>[2x]SMGEAICSALPTIPYHKLADLRYLSRGASGTVSSARHADWRVQVAVKHLHIHTPLLDSERKDVLREAEILHKARFSYILPILGICNEPEFLGIVTEYMPNGSLNELLHRKTEYPDVAWPLRFRILHEIALGVNYLHNMTPPLLHHDLKTQNILLDNEFHVKIADFGLSKWRMMSLSQSRSSKSAPEGGTIIYMPPENYEPGQKSRASIKHDIYSYAVITWEVLSRKQPFEDVTNPLQIMYSVSQGHRPVINEESLPYDIPHRARMISLIESGWAQNPDERPSFLKCLIELEPVLRTFEEITFLEAVIQLKKTKLQSV

RIPK2 is a caspase recruitment domain (CARD) containing kinase that has been implicated in nucleotide binding and oligomerization domain 1 and 2 (NOD1 and NOD2) signaling. NOD-RIPK2 interactions result in activation of nuclear factor κB (NF-κB) and mitogen-activated protein (MAP) kinase pathways to promote the transcription of pro-inflammatory cytokines. This signaling pathway potentially plays a crucial role in an array of pathological conditions including inflammatory bowel disease, Crohn’s disease and multiple sclerosis. Herein, we report the design of receptor-interacting protein kinase 2 (RIPK2) inhibitors based on pan-kinase inhibitor regorafenib that aim to engage basic activation loop residues Lys169 or Arg171.

We report development of CSR35 that displayed >10-fold selective inhibition of RIPK2 versus VEGFR2, the target of regorafenib. Two RIPK2 molecules were found in the asymmetric unit. As expected, CSR35 was bound to a DFG-out conformation and retained interactions characteristic of most type II inhibitors. The pyridine nitrogen and hydrogen of the amide formed hydrogen bonds with the hinge region (Met98). The urea was engaged in hydrogen bonds with the catalytic residue Glu66 and the backbone NH of Asp164 of the DXG motif. But most interestingly, one of the monomers revealed that Lys169 of the activation loop forms an ionic–ionic interaction with the carboxylate of the ligand and occupied a similar position as Arg171 in the previously reported structure. Engagement of Lys169 was consistent with the predicted result from sequence alignments and likely accounts for modest inhibitory activity differences between WT and R171C mutant RIPK2. Since the carboxylic acid will be deprotonated at pH 7.4, this functional group potentially forms an ionic–ionic interaction with the activation loop. Notably, CSR35 lacked significant activity in the in vitro enzymatic assay against the primary regorafenib target VEGFR2 (35.8 ± 2.6% inhibition at 20 μM), which does not have a basic residue in the same position as established by a published structure of VEGFR2 in the DFG-out conformation.> ASMKETNQKPYKETYGISHITRHDMLQIPEQQKNEKYQVPEFDSSTIKNISSAKGLDVWDSWPLQNADGTVANYHGYHIVFALAGDPKNADDTSIYMFYQKVGETSIDSWKNAGRVFKDSDKFDANDSILKDQTQEWSGSATFTSDGKIRLFYTDFS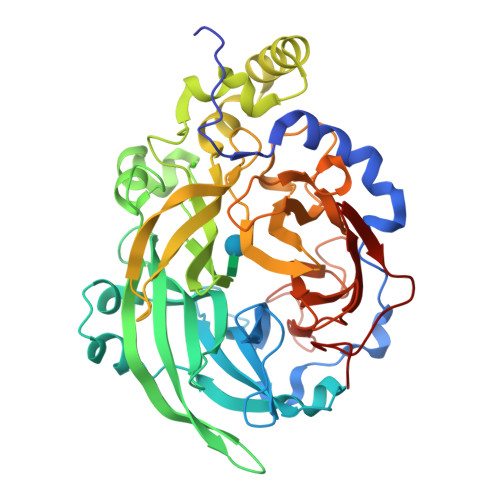GKHYGKQTLTTAQVNVSASDSSLNINGVEDYKSIFDGDGKTYQNVQQFIDEGNYSSGDNHTLRDPHYVEDKGHKYLVFEANTGTEDGYQGEESLFNKAYYGKSTSFFRQESQKLLQSDKKRTAELANGALGMIELNDDYTLKKVMKPLIASNTVTDEIARANVFKMNGKWYLFTDSRGSKMTIDGITSNDIYMLGYVSNSLTGPYKPLNKTGLVLKMDLDPNDVTFTYSHFAVPQAKGNNVVITSYMTNRGFYADKQSTFAPSFLLNIKGKKTSVVKDSILEQGQLTVNK> MTIAVTGSIATDHLMRFPGRFSEQLLPEHLHKVSLSFLVDDLVMHRGGVAGNMAFAIGVLGGEVALVGAAGADFADYRDWLKARGVNCDHVLISETAHTARFTCTTDVDMAQIASFYPGAMSEARNIKLADVVSAIGKPELVIIGANDPEAMFLHTEECRKLGLAFAADPSQQLARLSGEEIRRLVNGAAYLFTNDYEWDLLLSKTGWSEADVMAQIDLRVTTLGPKGVDLVEPDGTTIHVGVVPETSQTDPTGVGDAFRAG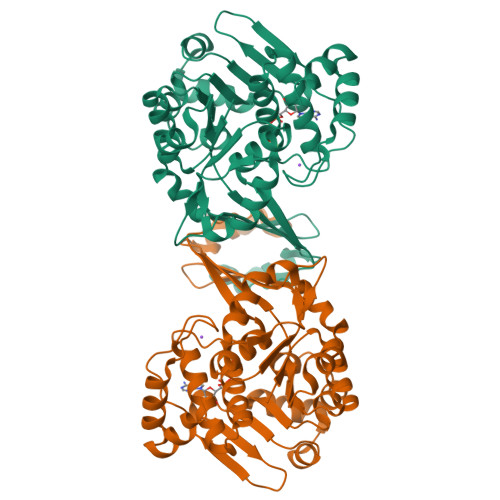FLTGRSAGLGLERSAQLGSLVAVLVLESTGTQEWQWDYEAAASRLAGAYGEHAAAEIVAVLA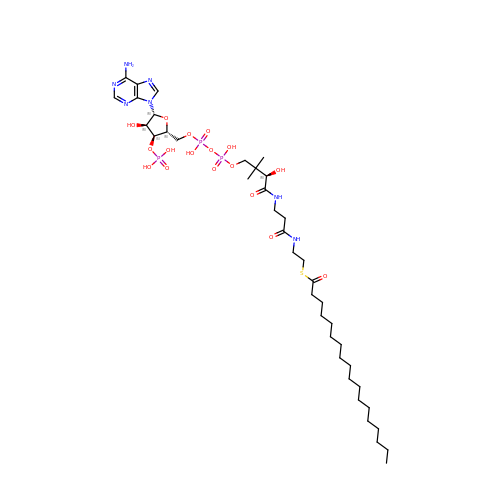STEAROYL-COENZYME A | C39 H70 N7 O17 P3 S | SIARJEKBADXQJG-LFZQUHGESA-N> TETTSFSITKFGPDQQNLIFQGDGYTTKERLTLTKAVRNTVGRALYSSPIHIWDSKTGNVANFVTSFTFVIDAPNSYNVADGFTFFIAPVDTKP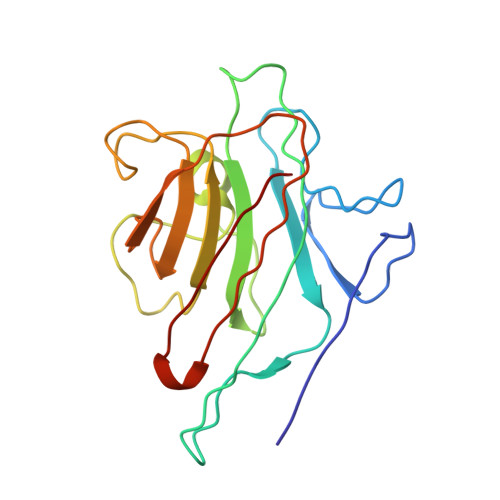QTGGGYLGVFNSKDYDKTSQTVAVEFDTFYNTAWDPSNGDRHIGIDVNSIKSINTKSWALQNGKEANVVIAFNAATNVLTVSLTYPN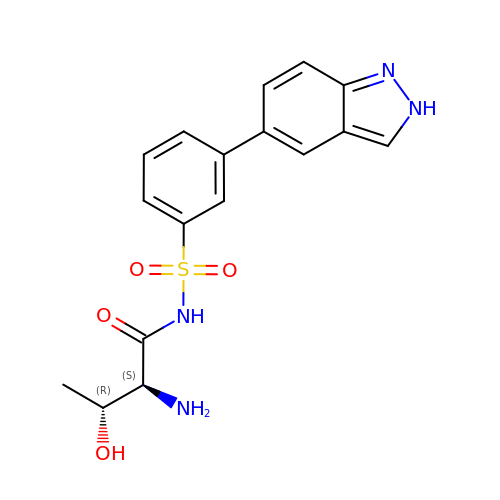N-{[3-(2H-indazol-5-yl)phenyl]sulfonyl}-L-threoninamide | C17 H18 N4 O4 S | RDKBQXPBHLCILS-HWPZZCPQSA-N>MARYYVLDLSEDFRRELRETLAEMVNPVEVHVFLSKSGCETCEDTLRLMKLFEEESPTRNGGKLLKLNVYYRESDSDKFSEFKVERVPTVAFLGGEVRWTGIPAGEEIRALVEVIMRLSEDESGLEDATKEALKSLKGRVHIETIIT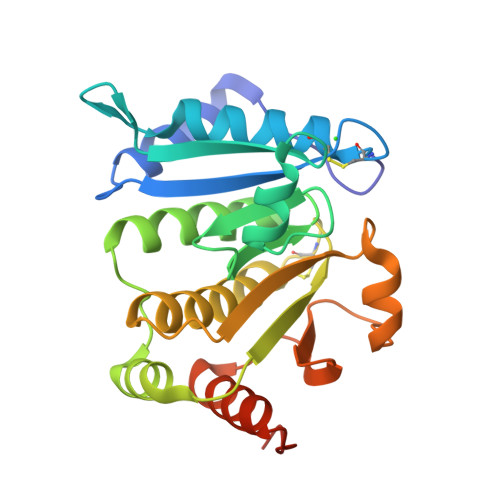PSCPYCPYAVLLAHMFAYEAWKQGNPVILSEAVEAYENPDIADKYGVMSVPSIAINGYLVFVGVPYEEDFLDYVKSAAEGRLTVKGPIRAGEAEEL[2x]> MEGSHHHHHHSQAQSKAQVLQSVAGQTLTVRCQYPPTGSLYEKKGWCKEASALVCIRLVTSSKPRTMAWTSRFTIWDDPDAGFFTVTMTDLREEDSGHYWCRIYRPSDNSVSKSVRFYL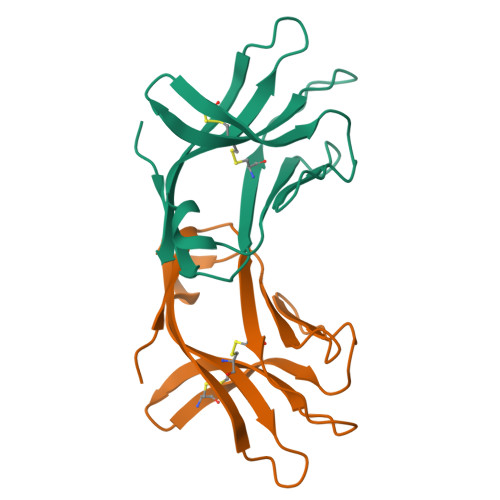VVS(2S)-2-{2-[(2-AMINOETHYL)AMINO]-2-OXOETHYL}-2-HYDROXYBUTANEDIOIC 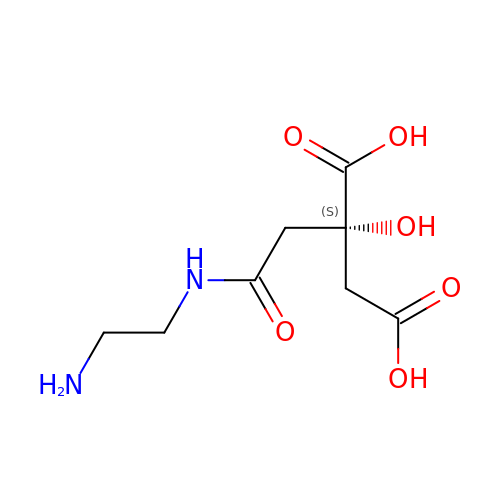ACID | C8 H14 N2 O6 | KQWWDTIPDRWKGZ-QMMMGPOBSA-N> MAYTSHLSSKTGLHFGRLSLRSLTAYAPNL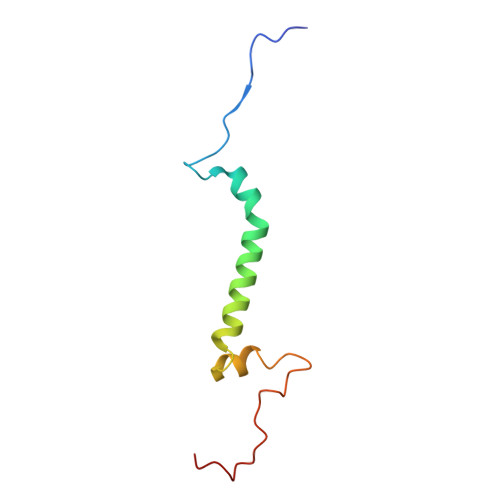MLWGGASMLGLFVFTEGWPKFQDTLYKKIPLLGPTLEDHTPPEDKPN> AYACSFPPGEIPGSKECLAEALQKHQGFKKK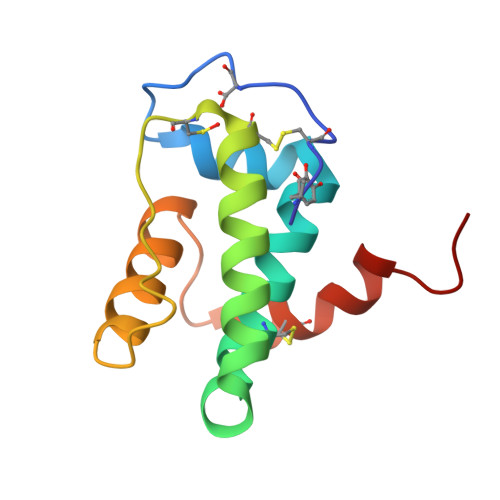SYALICAYLNYKEDAENYERAAEDFDSAVKCTGCKEGVDLHEGNPELIEEGFEKFLASLKIDRKALGSLCTLFQKLYAIPHN> MDPTDLSFSPDEINKLIETGLNTVEYFTSQQVTGTSSLGKNTIPPGVTGLLTNAAEAKIQESTNHQKGSVGGGAKPKKPRPKIAIVPADDKTVPGKPIPNPLLGLDSTPSTQTVLDLSGKTLPSGSYKGVKLAKFGKENLMTRFIEEPRENPIATSSPIDFKRGAGIPAGSIEGSTQSDGWEMKSRSLSGAIHPVLQSPLQQGDLNALVTSVQSLALNVNEILNTVRNLDSRMNQLETKVDRILSSQSLIQTIKNDIVGLKAGMATLEGMITTVKIMDPGVPSNVTVEDVRKTLSNHAVVVPESFNDSFLTQ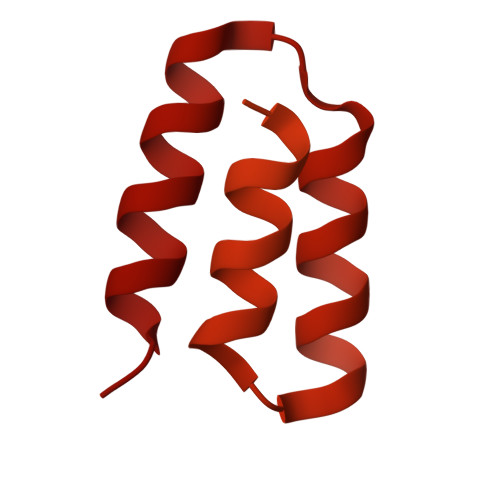SEDVISLDELARPTATSVKKIVRKVPPQKDLTGLKITLEQLAKDCISKPKMREEYLLKINQASSEAQLIDLKKAIIRSAI> MNNNKAE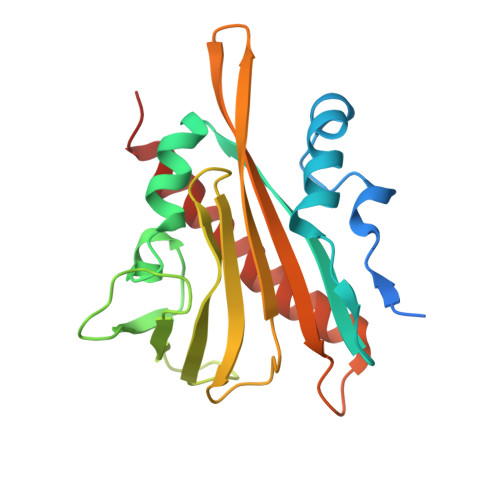ADTSSSMADPETRPTYTTHHLAIPSGVTQDEFDELKQSVVEFHTYQLSQNQCSSLLAQRIRAPNDVVWSIVRRFDQPQTYKHFIKSCSVSDNFTMAVGSTRDVNLISGLPAATSTERLDILDDDRQVLGISIIGGEHRLRNYRSVISVHGFNRDGAICTVALESYVVDVPEGNTEEDTRLFADTVVKLNLQKLVSVAESQVI> AAIDPNRIVALEWLPVELLLALGIV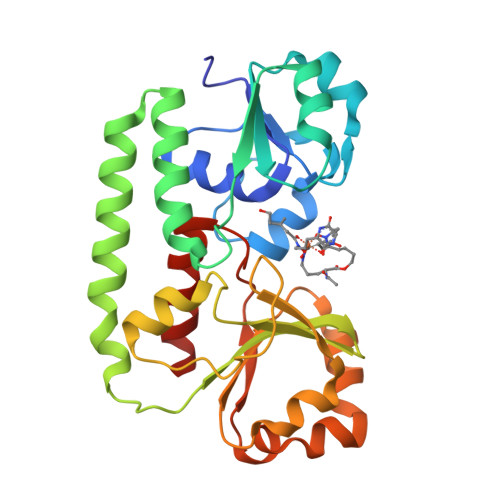PYGVADTINYRLWVSEPPLPDSVIDVGLRTEPNLELLTEMKPSFMVWSAGYGPSPEMLARIAPGRGFNFSDGKQPLAMARKSLTEMADLLNLQSAAETHLAQYEDFIRSMKPRFVKRGARPLLLTTLIDPRHMLVFGPNSLFQEILDEYGIPNAWQGETNFWGSTAVSIDRLAAYKDVDVLCFDHDNSKDMDALMATPLWQAMPFVRAGRFQRVPAVWFYGATLSAMHFVRVLDNAIGGKA>METSKEKTITSPGPYIVRLLNSSLNGCEFPLLTGRTLFVVGQSDALTASGQLPDIPADSFFIPLDHGGVNFEIQVDTDATEIILHELKEGNSESRSVQLNTPIQVGELLILIRPESEPWVPEQPEKLETSAKKNEPRFKNGIVAALAGFFILGIGTVGTLWILNSPQRQAAELDSLLGQEKERFQVLPGRDKMLYVAAQNERDTLWARQVLARGDYDKNARVINENEENKRISIWLDTYYPQLAYYRIHFDEPRKPVFWLSRQRNTMSKKELEVLSQKLRALMPYADSVNITLMDDVTAAGQAEAGLKQQALPYSRRNHKGGVTFVIQGALDDVEILRARQFVDSYYRTWGGRYVQFAIELKDDWLKGRSFQYGAEGYIKMSPGHWYFPSPL[24x];>MIRRYLYTFLLVMTLAGCKDKDLLKGLDQEQANEVIAVLQMHNIEANKIDSGKLGYSITVAEPDFTAAVYWIKTYQLPPRPRVEIAQMFPADSLVSSPRAEKARLYSAIEQRLEQSLQTMEGVLSARVHISYDIDAGENGRPPKPVHLSALAVYERGSPLAHQISDIKRFLKNSFADVDYDNISVVLSERSDAQLQAPGTPVKRNSFATSWIVLIILLSVMSAGFGVWYYKNHYARNKKGITADDKAKSSNE[24x]

The injectisome is a specialized bacterial organelle that utilizes a type III secretion system (T3SS) to translocate effector proteins from the bacterial cytosol directly into a eukaryotic host. Composed of >20 different proteins, the injectisome forms a syringe shaped nanomachine that spans both bacterial membranes and that of the infected host. The major structural unit of the injectisome is the basal body, composed of three highly oligomerized concentric rings spanning the bacterial inner membrane (IM) (PrgH and PrgK in the Salmonella enterica serovar Typhimurium SPI-1 T3SS)3–6 and outer membrane (OM)7 (InvG, a member of the secretin family of OM pores also found in the type II secretion system, type IV pili system, as well as the phage assembly system). To address this and further elucidate the structural basis for injectisome assembly and function, including that of the central needle component, we have conducted here a cryo-EM analysis of the assembled native needle complex resulting in 3D reconstructions of the IM and OM rings at resolutions permitting atomic model building (3.6 Å and 3.9 Å, respectively) and the 3D reconstruction of an isolated helical needle filament at 3.3 Å resolution.

The 24-fold features of the IM rings in the C1 reconstruction were clearly visible and further C24 symmetry averaging resulted in a reconstruction to 3.6 Å resolution (compared to 4.3 Å for the basal body IM rings; EMD-8398) allowing for refinement of the atomic structures of the periplasmic domains of PrgH171–364 and PrgK20–203. Consistent with the conserved dimensions of the IM rings between the needle complex here and that of the previous basal body reconstructions, the refined PrgH and PrgK ring atomic models determined from each overlap closely (overall Cα RMSD 0.7 Å) suggesting an inherently highly stable structure with no significant conformational change required in this region upon needle assembly. The N-terminal N0 and N1 domains, outer β-barrel and C-terminal surface exposed S domain conversely show very little structural difference between assembly states; as with the static IM ring components they appear to provide a highly stable scaffold or shell to buttress the inner conformational changes required for needle passage.>[2x]SLLRAVAHLRSQLWAHLPRAPLAPRWSPSAWCWVGGALLGPMVLSKHPHLCLVALCEAEEAPPASSTPHVVGSRFNWKLFWQFLHPHLLVLGVAVVLALGAALVNVQIPLLLGQLVEVVAKYTRDHVGSFMTESQNLSTHLLILYGVQGLLTFGYLVLLSHVGERMAVDMRRALFSSLLRQDITFFDANKTGQLVSRLTTDVQEFKSSFKLVISQGLRSCTQVAGCLVSLSMLSTRLTLLLMVATPALMGVGTLMGSGLRKLSRQCQEQIARAMGVADEALGNVRTVRAFAMEQREEERYGAELEACRCRAEELGRGIALFQG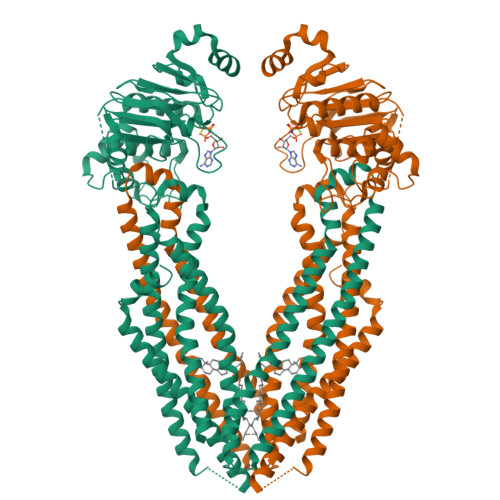LSNIAFNCMVLGTLFIGGSLVAGQQLTGGDLMSFLVASQTVQRSMANLSVLFGQVVRGLSAGARVFEYMALNPCIPLSGGCCVPKEQLRGSVTFQNVCFSYPCRPGFEVLKDFTLTLPPGKIVALVGQSGGGKTTVASLLERFYDPTAGVVMLDGRDLRTLDPSWLRGQVVGFISQEPVLFGTTIMENIRFGKLEASDEEVYTAAREANAHEFITSFPEGYNTVVGERGTTLSGGQKQRLAIARALIKQPTVLILDEATSALDAESERVVQEALDRASAGRTVLVIAHRLSTVRGAHCIVVMADGRVWEAGTHEELLKKGGLYAELIRRQALDAPRTAAPPPKKPEGPRSHQHKS> MAHHHHHHMEKTLSNAAIATESISNQALPSHYNYPNSLTLKNKYGITNHKDFTNKCAHDSAKAAINLRQEEPPKKFDSSYLKYLHKQLFKETFEWAGHTRDLPFTFADGTVGVMPEMIRSNWRTEQPIIFATGNKVQDGLKNIDKMLIEKNNLQGLSHKEFIENIAEIFACLNYTHPFREGNGRTQRIFCEKLAQAAGYYLDFSVVTKERMSEASITAAQDSNLEPMKKLFDDISNPIKTAVLKECINSLKNIDHKNINDCIIVAADKGLTYKGIYTDNSPDSIILKTDNIYIICSKNDLAPEQLKTLKLGDECTITVPMKQNIENTLIPKEKLPPLTKNAIIENIKKDTLIQAKLRQVTHLSKLVYGSSKILNNQLELINTNQKSGEQLSAQITSSPQSISKLAGIKIFGMKNSMRKKAEDNIIKLANSIKSYGSAVKNVETTMIQQHKSEQKRLSKTVKLPSTKLQNILNLPEEKQKEVLLEEKSLASSIGKELTDFISSLNARLSPSERKMILESNHQQFAKNVGISESQAETIIKTAQKAKEVYQKMQKPAVDLTKHLIVSG

Proteins containing a FIC domain catalyze AMPylation and other post-translational modifications (PTMs). Among these, Bartonella effector proteins (Beps) comprise a particularly diverse ensemble of FIC domains that subvert various host cellular functions. The FIC fold comprises eight conserved α-helices and encompasses a characteristic active site loop between helices α4 and α5 that forms most of the catalytic center and the substrate binding pocket. Additionally, FIC domains generally contain a β-hairpin between helix α2 and helix α3 that is referred to as the “flap” and mediates docking of a target segment in extended conformation via β-strand augmentation.

The structures of Bhe_BepA, Bcl_Bep1, Bqu_BepC, and Btr_BepC exhibit all features defining a FIC AMP transferase as described in the first chapter and elsewhere. So far, it has been shown that Bep1 AMPylates Rac-subfamily GTPases, Bep2 AMPylates the host intermediate filament protein vimentin, and BepA causes the AMPylation of two unknown host proteins of ca. 40–50 kDa size. All members of branch 1 are predicted to catalyze AMP transfer (indicated in green in the cladogram). This has been verified for Bro_Bep1, which AMPylates the switch 1 loop of small GTPases. Very recently, it has been shown that small GTPases of the Rac-subfamily are the target for Bep1 and that two residues in the extended flap are critical for the exquisite target specificity. With the use of modeling, this finding was rationalized by suggesting that they form two salt-bridges with Rac-subfamily specific residues. Bcl_Bep1 FIC were grown from a solution of 10% w/v PEG 20,000, 20% v/v PEG MME 5500, 0.1 M MOPS/HEPES-Na, pH 7.5, and 0.02 M each of sodium formate, ammonium acetate, trisodium citrate, sodium potassium L-tartrate, and sodium oxamate. Data for Bqu_BepC FIC with ADP, Bcl_Bep1 FIC, and B11C_Bep8 FIC were collected at 100 K on a Rayonix MX-225 detector at a wavelength of 0.9786 Å on beamline 21-ID-F at the Advanced Photon Source (APS, Argonne, IL, USA).N-[(1S)-2-hydroxy-1-phenylethyl]-3-methoxy-4-(1H-pyrazol-4-yl)benzamide | C19 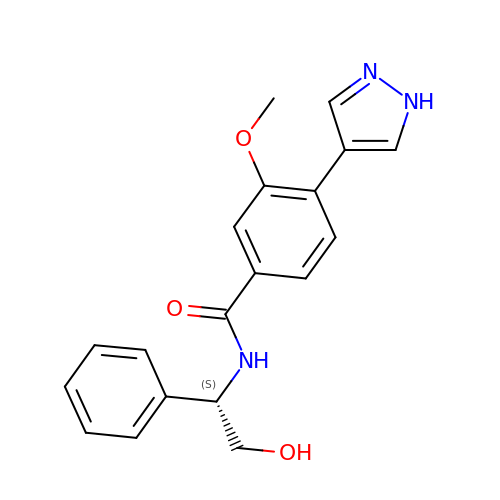H19 N3 O3 | CXWOMMUYWIPPCD-QGZVFWFLSA-N>MSFTPANRAYPYTRLRRNRRDDFSRRLVRENVLTVDDLILPVFVLDGVNQRESIPSMPGVERLSIDQLLIEAEEWVALGIPALALFPVTPVEKKSLDAAEAYNPEGIAQRATRALRERFPELGIITDVCLCPFTTHGQDGILDDDGYVLNDVSIDVLVRQALSHAEAGAQVVAPSDMMDGRIGAIREA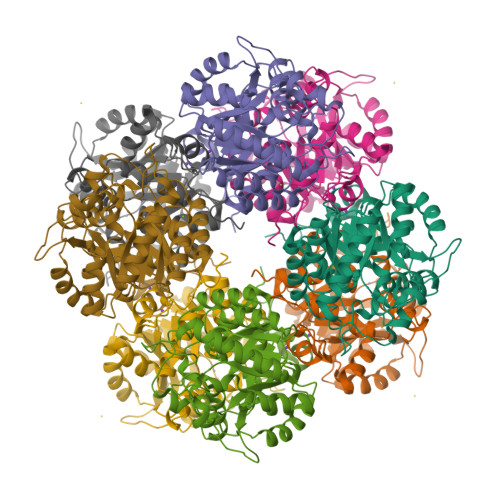LESAGHTNVRVMAYSAKYASAYYGPFRDAVGSASNLGKGNKATYQMDPANSDEALHEVAADLAEGADMVMVKPGMPYLDIVRRVKDEFRAPTFVYQVSGEYAMHMGAIQNGWLAESVILESLTAFKRAGADGILTYFAKQAAEQLRRGR[2x]>TLHKERRIGRLSVLLLLNEAEESTQVEELERDGWKVCLGKVGSMDAHKVIAAIETASKKSGVIQSEGYRESHALYHATMEALHGVTRGEMLLGSLLRTVGLR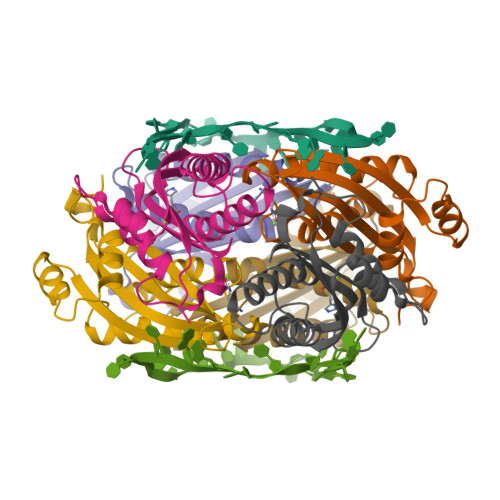FAVLRGNPYESEAEGDWIAVSLYGTIGAPIKGLEHETFGVGINHI[3x]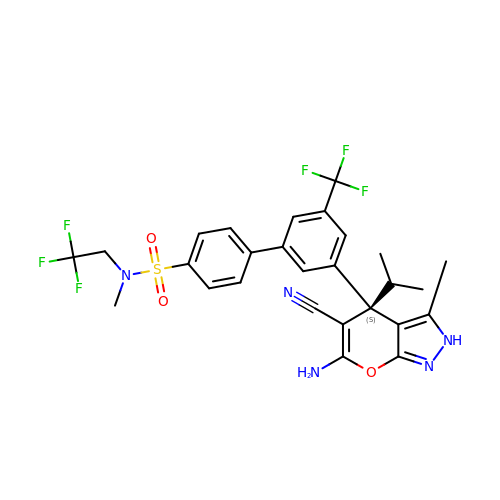4-[3-[(4~{S})-6-azanyl-5-cyano-3-methyl-4-propan-2-yl-2~{H}-pyrano[2,3-c]pyrazol-4-yl]-5-(trifluoromethyl)phenyl]-~{N}-methyl-~{N}-[2,2,2-tris(fluoranyl)ethyl]benzenesulfonamide | C27 H25 F6 N5 O3 S | IWWMJNMFKYGJIC-SANMLTNESA-N In the gliding bacterium, Mycoplasma mobile, a dimeric F1-like ATPase forms a chain structure within the cell, which is proposed to drive the gliding motility. The motor is formed by dimerized F1-like ATPases with unique bridge structures and is referred to as a twin motor. The F1-like ATPase unit associated by two subunits GliD and GliE was named G1-ATPase as an R1 domain of rotary ATPases. Structural features of the ATPase displayed strong similarities to F1-ATPase, suggesting a rotation based on the rotary catalytic mechanism.

The twin motor exhibited a rectangular structure with dimensions of approximately 350 × 250 × 150 Å and at least 24 polypeptide chains with a total mass of approximately 1.5 MDa. Notably, the two F1-like ATPases were inclined to each other by approximately 5° and formed a dimer with pseudo-twofold rotational symmetry and several accessories. The F1-like ATPase comprised a hexameric ring of two alternating subunits and a central shaft subunit, identified as MMOBs 1660, 1670, and 1630, respectively. In the hexameric ring, nucleotide-derived densities were observed at five of the six subunit interfaces, despite the isolation and analysis of samples under nucleotide free condition, indicating the presence of endogenous nucleotides as reported in F1-ATPase. The subunit attached to α, forming a “bridge” between two α3β3γ subcomplexes, was identified as MMOB1620 and named GliD in the present study. The three densities protruding from the G1-ATPase dimer were identified as MMOB4530, which was previously annotated as PGK. In addition, at the interface of the two G1-ATPase monomers, the N-terminal regions of G1-β3 and G1-β6 interacted with the NBDs of G1-α6 and G1-α3 of another G1-ATPase monomer, respectively. These interactions suggest that the β-specific N-terminal region plays a role in the incorporation of PGK into the twin motor and stabilization of the ATPase dimer. GliD contained a globular domain and an N-terminal long α-helix (H2), which was only visualized in the dimer. The two H2 helices in the GliD dimer aligned parallel to each other across the H20–H25 region of α, GliE, β-NTD, and β-CTD. The GliE subunit, which is bound to only one side of the dimeric G1-ATPase, creates asymmetry in the twin motor structure and may contribute to the unidirectional nature of the gliding motility.

>[6x]MTTNNLTELEILNIKKYLKTVNLNTLRAYARRNVKDFSEKLIKVKVIEKIVEHDKKFDNIEDSIFVQISSQFGVNFETILDGSFFLGQKAAKAMPKTFDTKIISETKSVQKFEEVKFATSSKTEKIISEEKEILHLIEQSKRDRDFIDNFSKILEEKNLTEEHQHMSCQVCYDHEKKHSDHNEKYATEHCDACVYHDFSDLDPEFVASTYTEEEIIHNLLFKLYSVEQLALFTIDQLNALLFARGLGLEKNKVRAIKSLLTLQTSYEFMEKSQAALLPKVSFNPTNPLKPIEEKEFTIFGEIVEIRSQVYKIRIDKAEEEVLPKVIFYADVNGKEIQLEVADIFDKNLVSTFVLGNETGLKIGTKVKSKNQSYAIKISKRLLGRVIDPIGKILDDSIATPVHGNMYAPLEMQHDSEATRYVVSPKNAILETGIKVIDVLLPIPKGGKTGLLGGAGVGKTVIVQELINAFIKFHDGVSVFAGIGERIREGHELWKEAEALGFLNKTAFIFGQMNESPGLRFRSGISGVKVAEYFRNNLGKSVLLFMDNIFRYVQAGSEISSLLEKTPSAVGYQPTLFSEMGQLQERINSTKDGDITSIQAMYIPADDFTDPAAVAAFAHFDSTIILSRQLAAEGVYPAIDPLESNSKMLSIKYTSREHLDIAKKTVQTLEKTKTLEDIINILGFDALSEDDKKVVEVGRRLKWFLTQPFVVAEKFSGVPGKFVRLKDSLKGIKTILDGDLNHIPVSYFSFVGVVEEIIEKFNLDAKKEALKNELEQNQKDLASII;>[6x]MKNLKITAIKDNLIFVEGEHQFSFLEIIKFSDKVEGVVLKANDRSAIVAILNEDKDLNLTVGSLAEATGELYKIPIYDNYLGSIINVLGESLVKQYERTNVALDKKYVFTEAQPIFTRSAVNEPLVTGITVVDGVLPVGRGQKELIIGDRGTGKTAIALNAMLAQENTDVINIFIAIGKKRDEIVEIYGTFKKHNILHKSIIVSAASDDAVAARYLAPYAGMAIAEFFQQIGKDVLVVMDDLTNHADAYRELSLLAGIAPAREAYPGDIFYVHSSLLERGGKYGPEFGGGSITILPIAQTLAGDISGYIPTNLISITDGQIYTSAKLFNEGTRPAIDVNLSVSRLGSAAQSKFMAFASSGLKKIYTEYKYLKRLSSFSSKISNRDLETLQKGKAFESLIDQAEYEVIDYETSAILFLLLKKGFLNFYTEKTEALKVIIGVIKVFLAKDVLGRKMRAILVEHGIDSIVWNLYLNHMILPLLKYHLLSELQYLATNREFIKKFKDIRNDGRILLAYERKGYERGIAYDYK;>MKRKDVEEKKQNLDFYHNYIDISKIKVLQKLNEEIASLNMLKLQKGESHYLLNRIINKWFPHNSNIYHELHHENDRKELYILIDPKKLDLFSEALLRKLSQTVKERIRPDKDFVITVGTNVDNIARQLNLNIIDHYDLDLFNQIDDFANRIGELVDVGLNNKIFNYVSLLIAQSSTKNNGGLVQERIVPFNTKNIKVWNESNQDENGMPIVSEENEVEIMSYAKTLRNINFKKHTWLPNINTFYEQFVKSVFKQELFEFKSISVIEELKIELQLLDEKKKRLEEQKKELILKWNRARKEEATLQSTLLFSAFKVKNQKSTRDEILRLSKGKNRNGA[2x];>[3x]MKKTLDQISLKNKKVIIRVDFNVPIVNGIVTSNKRIEAVIPTIKKVVNEGGKAILMSHLGRVKSEEDLKKKSLAPVVEILVNLLGMPITFVPATNGTELEETINSMKSGEIVMMENTRFEDLNNDAESSNNPDLGMYWASLGDVFINDAFGTVHRKHASNVGISTYIAESGIGYLVEKEIKNLDKALSRPERPIVAILGGAKVSDKIGVLNNLLKYVDKIIIGGAMAYTFLAAQGIGIGKSLVEEDKIDLAREYLKNNLDKFVLPIDYALAKDFEDVKPFYNLENTLEIPNGYMGLDIGPKSIEVFKKYIKDAKTILWNGPLGVTEFKYFKEGTKAIAKAITELKGNVYTVVGGGDSVAIIEELGLDRRFSHVSTGGGATLEFLEGKELPGIQAIQNEGELGRTKEEIFSILTQNSEEVLHEHTAAFSTSEVEPANEEFPSEYNDSNSQTYFSNEVENDEDFLLNTNDFPTREASFPNEVKTEEIILNENDDEFDIEDEELDSLPNDDIKF;>[6x]MKKTDKNQTGKEIMKKELLIKTNEQDINLAPKSQSTSKKLSNTWNYEELINQTKEIDVNSKIVKTELEYVEEDSRLRKEKIELIQKNYDNLNAKPLVGVDLYESYSLVLNKSAWNYNEIIQRDTQLTILDMALQVHLFLYEGKIIDIAHIQKIIKTFVLNVFAKIIKGVPIVLNPIIIFDSVRFDKSKILPVAVANPKLMPPLGVQDWDTIVDEDEEIKKIVSTFIKLLENALTVGHEVEFFQDTLLVRNVDGITSLYVSEKAAQVFNNSVIDQIMPEKPKYEALEDPFSNKK;> MTKNIFANKIANQKAYFKRDIKTVHTFLGRVNYIQRASKFNDEKRVFRPLQIELSGTNEIVDIYLEATTYISKKALDEIRQNSYIFLEAKWLPESNFLNNPLFEIQNIVIEN4-azanyl-6-[[(1~{S})-1-(6-fluoranyl-3-phenyl-4-piperazin-1-ylcarbonyl-quinolin-2-yl)ethyl]amino]pyrimidine-5-carbonitrile | C27 H25 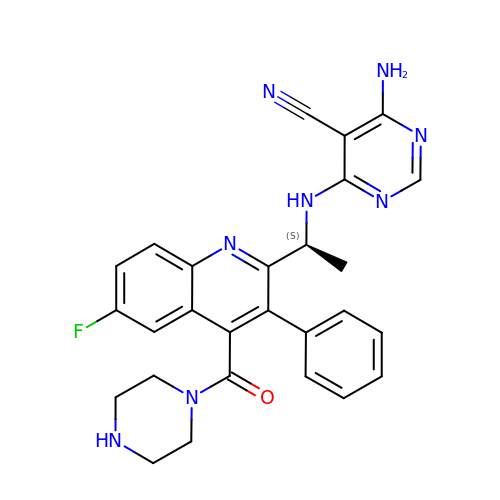F N8 O | QPRMAEKTXODJGJ-INIZCTEOSA-N[(2~{R},3~{S},4~{S},5~{R})-3,4-bis(oxidanyl)-5-[3-[4-(4-oxidanylbutyl)-1,2,3-triazol-1-yl]propyl]oxan-2-yl]methyl ~{N}-[(2~{S})-2-azanyl-4-methyl-pentanoyl]sulfamate 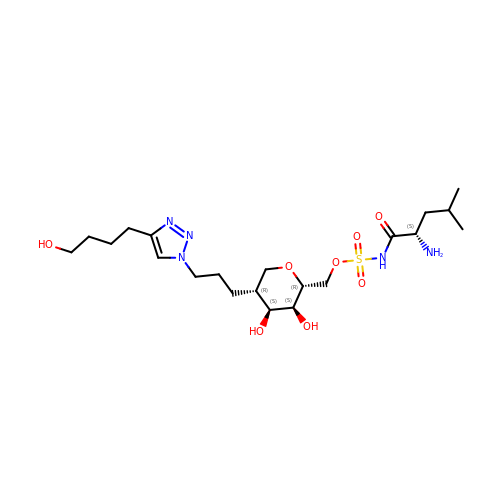| C21 H39 N5 O8 S | GYRXQACHPUUHBN-MTEHYEEQSA-N2'-DEOXYCYTIDINE-5'-MONOPHOSPHATE 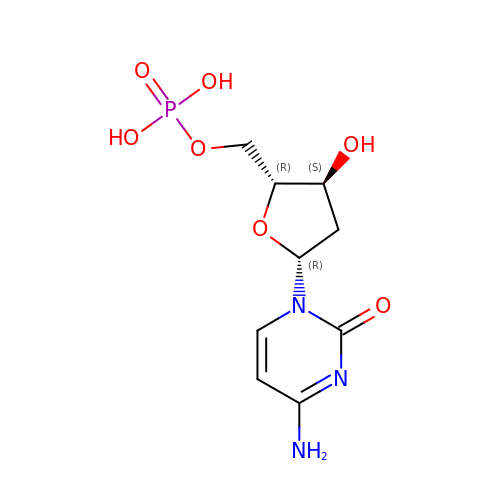| C9 H14 N3 O7 P | NCMVOABPESMRCP-SHYZEUOFSA-N> ELQEADGQCPVDRSLLKLKMVQVVFRHGARSPLKPLPLEEQVEWNPQLLEVPPQTQFDYTVTNLAGGPKPYSPYDSQYHETTLKGGMFAGQLTKVGMQQMFALGERLRKNYVEDIPFLSPTFNPQEVFIRSTNIFRNLESTRCLLAGLFQCQKEGPIIIHTDEADSEVLYPNYQSCWSLRQRTRGRRQTASLQPGISEDLKKVKDRMGIDSSDKVDFFILLDNVAAEQAHNLPSC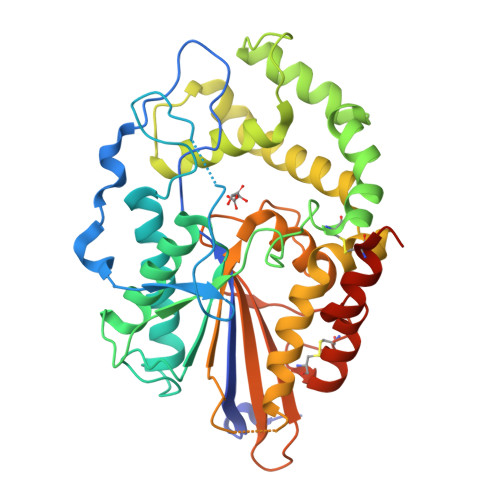PMLKRFARMIEQRAVDTSLYILPKEDRESLQMAVGPFLHILESNLLKAMDSATAPDKIRKLYLYAAHDVTFIPLLMTLGIFDHKWPPFAVDLTMELYQHLESKEWFVQLYYHGKEQVPRGCPDGLCPLDMFLNAMSVYTLSPEKYHALCSQTQVMEVGNEE>ASASTPHALLLISIDGLRADMLDRGITPNLSHLA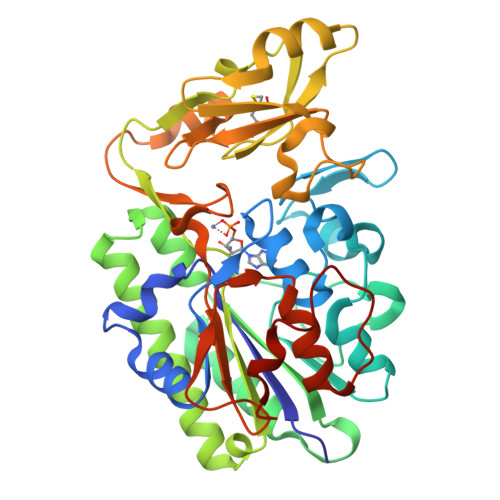REGVRARWMAPSYPSLTFPNHYTLVTGLRPDHHGIVHNSMRDPTLGGFWLSKSEAVGDARWWGGEPVWVGVENTGQHAATWSWPGSEAAIKGVRPSQWRHYQKGVRLDTRVDAVRGWLATDGAQRNRLVTLYFEHVDEAGHDHGPESRQYADAVRAVDAAIGRLLAGMQRDGTRARTNIIVVSDHGMAEVAPGHAISVEDIAPPQIATAITDGQVIGFEPLPGQQAAAEASVLGAHDHYDCWRKAELPARWQYGSHPRIPSLVCQMHEGWDALFPDKLAKRAQRGTRGSHGYDPALPSMRAVFLAQGPDLAQGKTLPGFDNVDVYALMSRLLGIPAAPNDGNPATLLPALRMPPAPDAR[2x]>MSVKIGINGFGRIGRLAFRRILELGEKSSDIEVVAINDLTSPALLAHLLKYDSTHGTLNADVSATDDSIVVNGKNYRVYAEPQAQNIPWVKNDGVDFVLECTGFYTSKAKSQAHLDAGAKRVLISAPAGSDLKTIVYNVNDDILTADDRIVSAGSCTTNCLAPLAFFENKEFGIKVGTMTTIHAYTSTQMLLDGPVRGGNFRAARAAGVNTIPHSTGAAKALGLVIPELNGKLQGHAQRVGVVDGSLTELVAILDKKVTADEVNAAIKKHTEGNESFGYNDDEIVSSDVIGT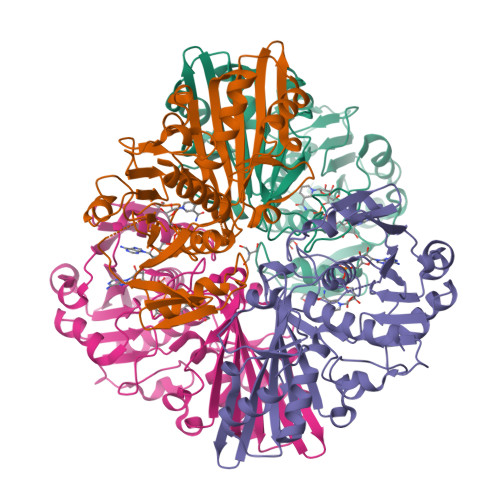TFGSIFDPTQTEVTSDGDNQLVKTVAWYDNEYGFTCQMVRTLLKFATL[4x]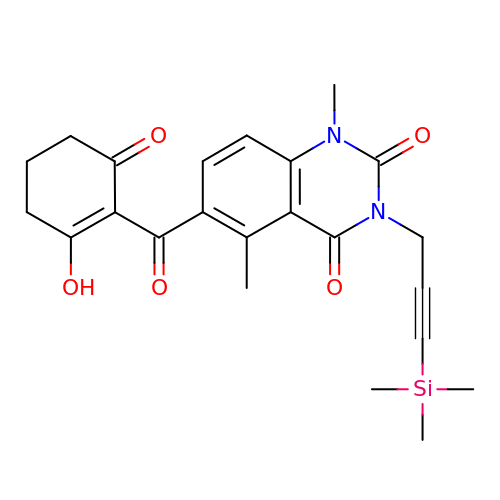1,5-dimethyl-6-(2-oxidanyl-6-oxidanylidene-cyclohexen-1-yl)carbonyl-3-(3-trimethylsilylprop-2-ynyl)quinazoline-2,4-dione | C23 H26 N2 O5 Si | YTIYFYIVVDHCTC-UHFFFAOYSA-N9-ethyl-~{N}-[(4-ethylsulfonylphenyl)methyl]-6-propan-2-yloxy-carbazole-3-carboxamide | C27 H30 N2 O4 S | 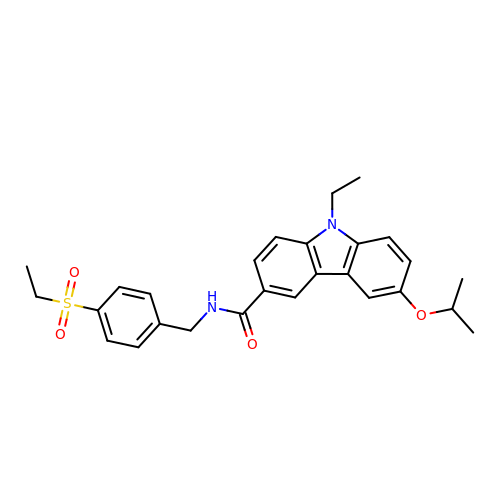ATOIOYVURMTRSQ-UHFFFAOYSA-N> MSRLDKSKVINSALELGNEVGIEGLTTRKLAQKLGVEQPTLYWHVKNKRALLDALAVEILARHHDYSLPAAGESWQSFLRNNAMSFRRALLRYRDGAKVHLGTRPDEKQYDTVETQLRFMTENGFSLRDGLYAISAVSHFTLGAVLEQQEHTAALTDRPAAPDENLPPLLREALQIMDSDDGEQAFL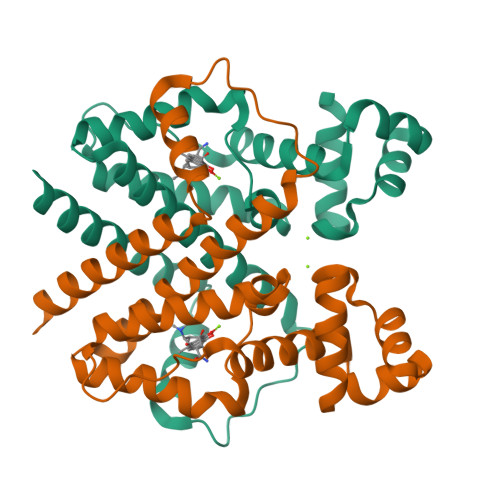HGLESLIRGFEVQLTALLQIV> MEGERKNNNKRWYFTR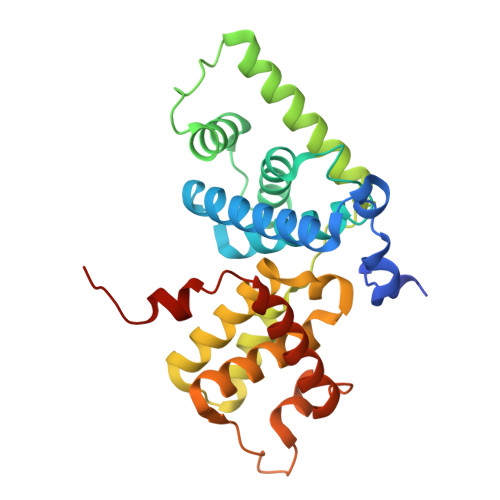EQLENSPSRRFGVDPDKELSYRQQAANLLQDMGQRLNVSQLTINTAIVYMHRFYMIQSFTQFPGNSVAPAALFLAAKVEEQPKKLEHVIKVAHTCLHPQESLPDTRSEAYLQQVQDLVILESIILQTLGFELTIDHPHTHVVKCTQLVRASKDLAQTSYFMATNSLHLTTFSLQYTPPVVACVCIHLACKWSNWEIPVSTDGKHWWEYVDATVTLELLDELTHEFLQILEKTPNRLKRIWNWRACEAA> MKLLKYLCIGISALSILSCSDWTSEEREVFENQEGMHRLIPLIEAQTEEDLTPTMREYFAQIREYRKTPHVKGFGWFGNWTGKGNNAQNYLKMLPDSVDFVSLWGTRGYLSDEQKADLKFFQEVKGGKALLCWIIQDLGDQLTPKGLNATQYWVEEKGQGNFIEGVKAYANAICDSIEKYNLDGFDIDYQPGYGHSGTLANYQTISPSGNNKMQVFIETLSARLRPAGRMLVMDGQPDLLSTETSKLVDHYIYQAYWESSTSSVIYKINKPNLDDWERKTIITVEFEQGWKTGGITYYTSVRPELNSMEGNQILDYATLDLPSGKRIGGIGTYHMEYDY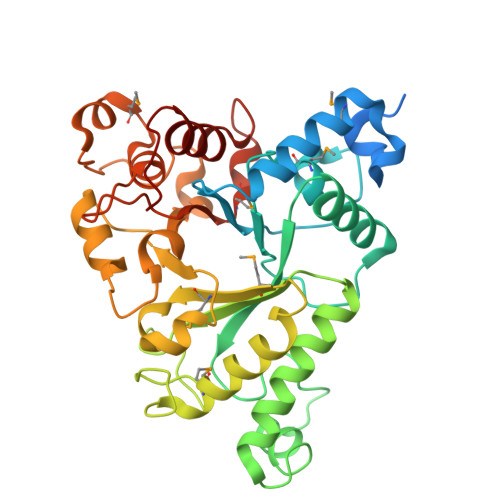PNDPPYKWLRKALYFGNQVYPGKFD> MARAKLKNSPSESNSHVKTVPPATTEDVRGVSPLLPARRMGSLGSDVGQRPHAEDFSMDSSFSQVQVEFYVNENTFKERLKLFFIKNQRSSLRIRLFNFSLKLLTCLLYIVRVLLDNPEEGIGCWECEKQNYTLFNQSTKINWSHIFWVDRKLPLWAVQVSIALISFLETMLLIYLSYKGNIWEQIFRISFILEMINTVPFIITIFWPPLRNLFIPVFLNCWLAKYALENMINDLHRAIQRTQSAMFNQVLILICTLLCLVFTGTCGIQHLERAGEKLSLFKSFYFCIVTFSTVGYGDVTPKIWPSQLLVVIMICVALVVLPLQFEELVYLWMERQKSGGNYSRHRAQTEKHVVLCVSSLKIDLLMDFLNEFYAHPRLQDYYVVILCPTEMDIQVRRVLQIPLWSQRVIYLQGSALKDQDLMRAKMDNGEACFI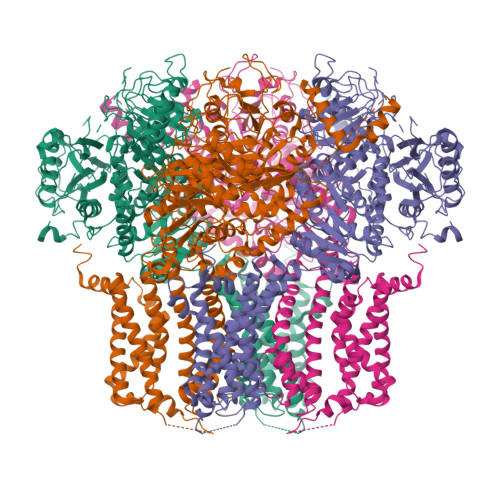LSSRNEVDRTAADHQTILRAWAVKDFAPNCPLYVQILKPENKFHVKFADHVVCEEECKYAMLALNCVCPATSTLITLLVHTSRGQEGQESPEQWQRMYGRCSGNEVYHIRMGDSKFFMEYEGKSFTYAAFHAHKKYGVCLIGIRREENKSILLNPGPRHIMAASDTCFYINITKEENSAFIFKQAEKQKKKGFAGRGTYDGPSRLPVHSIIASMGTVAMDLQNTECRPTNSSKLALPAENGSGNRRPSIAPVLELADTSSLLPCDLLSDQSEDEMTQSDEEGSAVVEYVKGYPPNSPYIGSSPTLCHLLPEKAPFCCLRLDKGCKHNSFEDAKAYGFKNKLIIVSAETAGNGLYNFIVPLRAYYRSRKELNPIVLLLDNKPEHHFLEAICCFPMVYYMEGTIDNLDSLLQCGIIYADNLVVVDKESTMSAEEDYMADAKTIVNVQTMFRLFPSLSIITELTHPSNMRFMQFRAKDSYSLALSKLEKKERENGSNLAFMFRLPFAAGRVFSISMLDTLLYQSFVKDYMITITRLLLGLDTTPGSGYLCAMKITEDDLWIRTYGRLFQKLCSSSAEIPIGIYRTESHMFATSEPHDIRAQSQISINVEDCEDTKDVKEHWGIKTGHHRNSCSSDQSEHPLLRRKSMQWARRLSRKGNKHSGKTAEWISQQRLSLYRRSERQELSELVKNRMKHLGLPTTGYDEMNDHQNTLSYVLINPPPDTRLELNDIVYLIRSDPLAHVANDGHSRKSSCSNKLGPCNPETRDETQL>GSMRGKVSLEEAFELPKFAAQTKEKAELYIAPNNRDRYFEEILNPCGNRLELSNKHGIGYTIYSIYSPGPQGWTERAECEEYARECNDYISGEIANHKDRMGAFAALSMHDPKQASEELTRCVKELGFLGALVNDVQHAGPEGETHIFYDQPEWDIFWQTCVDLDVPFYLHPEPPFGSYLRNQYEGRKYLIGPPVSFANGVSLHVLGMIVNGVFDRFPKLKVILGHLGEHIPGDFWRIEHWFEHCSRPLAKSRGDVFAEKPLLHYFRNNIWLTTSGNFSTETLKFCVEHVGAERILFSVDSPYEHIDVGC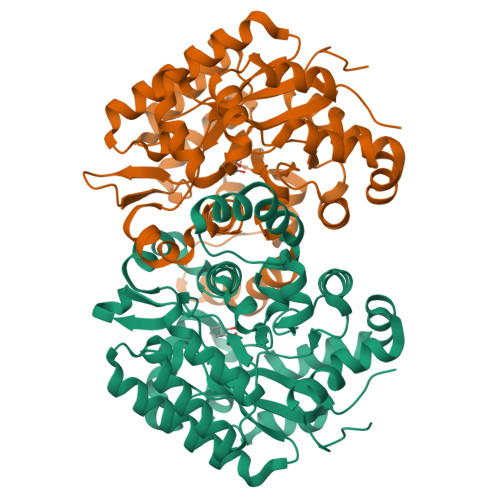GWYDDNAKAIMEAVGGEKAYKDIGRDNAKKLFKLGKFYDSEA[2x]>LAAALAQ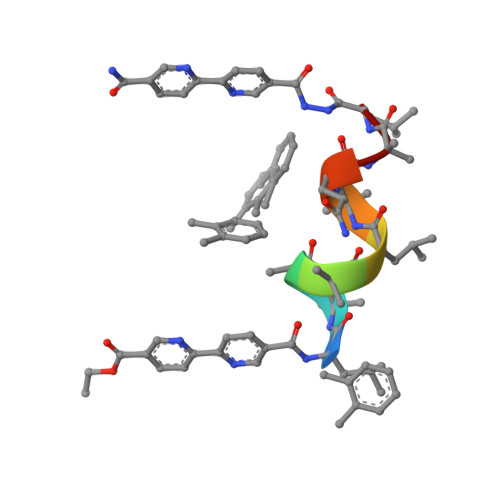AL[2x]>[2x]MGSSIKKISFVGIFSALATLVMFLEFPIFPQASFLKYDPSEIPALIVSFLLGPGVGMFVVLV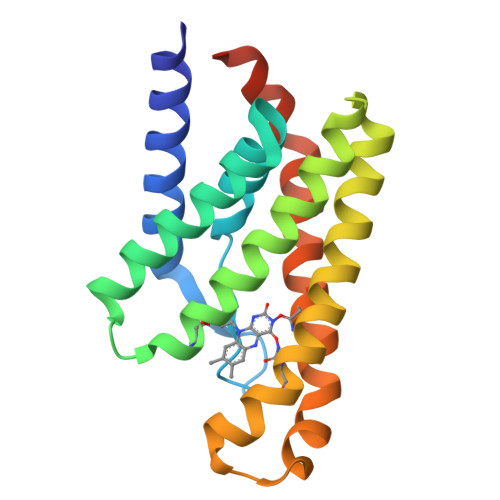KDILFFLMKSGDPVGIAMNAVLGMSFVGIAGLIYHRNKSRATAIKGMIVATLFATAFALGLNALIVPLYFEAPFELYLKFFPFILAFNLVKFGIDSVVTFFVYKKVSSILKLSNSLVPR> MNKPVIEGYKVSGYILPDFSFDATVAPLVKAGFKVEIVGTELYAVTDANGYFEITGVPANASGYTLKISRATYLDRVIANVVVTGDTSVSTSQAPIMM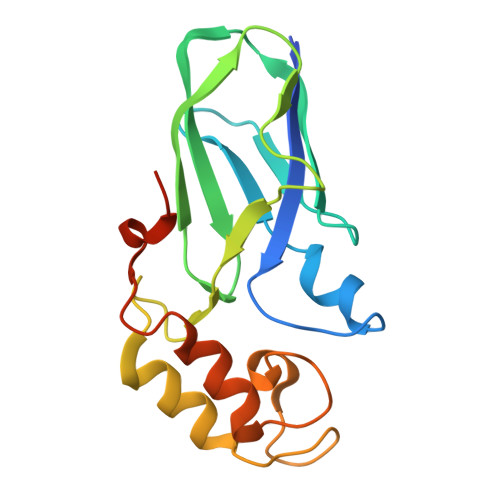WVGDIVKDNSINLLDVAEVIRCFNATKGSANYVEELDINRNGAINMQDIMIVHKHFGATSSDYDAQLEHHHHHH>GSNQKAVILDEQAIRRALTRIAHEMIERNKGMNNCILVGIKTRGIYLAKRLAERIEQIEGNPVTVGEIDITLYRDDLSKKTSNDEPLVKGADIPVDITDQKVILVDDVLYTGRTVRAGMDALVDVGRPSSIQLAVLVDRGHRELPIRADYIGKNIPTSKSEKVMVQLDEVDQNDLVAIYENEK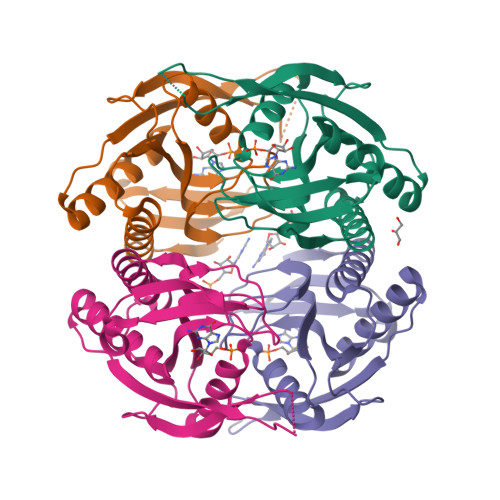[4x]>LEEKKVCQGTSNKLTQLGTFEDHFLSLQRMFNNCEVVLGNLEITYVQRNYDLSFLKTIQEVAGYVLIALNTVERIPLENLQIIKGNMYYENSYALAVLSNYDANKTGLKELPMRNLQEILHGAVRFSNNPALCNVESIQWRDIVSSDFLSNMSMDFQNHLGSCQKCDPSCPNGSCWGAGEENCQKLTKIICAQQCSGRCRGKSPSDCCHNQCAAGCTGPRESDCLVCRKFRDEATCKDTCPPLMLYNPTTYQMDVNPEGKYSFGATCVKKCPRNYVVTDHGSCVRACGADSYEMEEDGVRKCKKCEGPCRKVCNGIGIGEFKDSLSINATNIKHFKNCTSISGDLHILPVAFRGDSFTHTPPLDPQELDILKTVKEITGFLLIQAWPENRTDLHAFENLEIIRGRTKQHGQFSLAVVSLNITSLGLRSLKEISDGDVIISGNKNLCYANTINWKKLFGTSGQKTKIISNRGENSCKATGQVCHALCSPEGC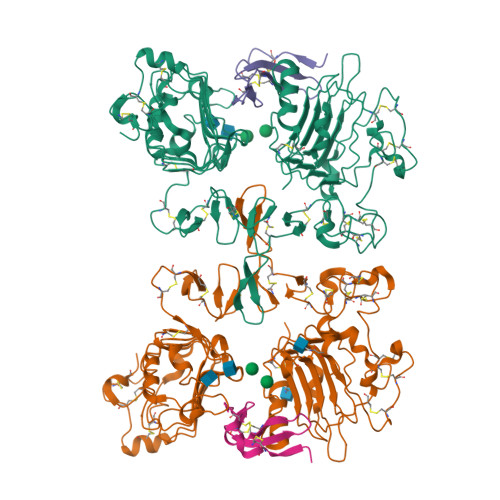WGPEPRDCVSH[2x];>[2x]VSITKCSSDMNGYCLHGQCIYLVDMSQNYCRCEVGYTGVRCEHFFLTV>EVLFQGPKE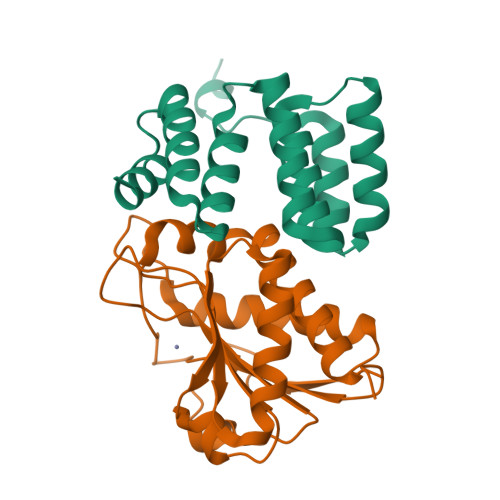DNIYNKLIKDDMTSGNYDNAQNIAKQTINKNYADDQTYYLSGMIMATINSKSEGMTEWERGLRMFPKSGLLNFELAIANRSLNDDEKALKYVRKALNADPKNTDYINLEKELT[2x];>[2x]MLQGKTIVLDPGHGGSDQGASSNTKYKSLEKDYTLKTAKELQRTLEKEGATVKMTRTDDTYVSLENRDIKGDAYLSIHNDALESSNANGMTVYWYHDNQRALADTLDATIQKKGLLSNRGSRQENYQVLAQTKVPAVLLELGYISNPTDETMIKDQLHRQILEQAIVDGLKIYFSA>MAAQHGAPPSARSPRFGVNYTPSNGWFHHWLDFDLDAVRADLDSVAALGFDHVRVFPLWPVFQPNRTLIRPRAVEQLAALTDAAGERGLDVNVDGLQGHLSSFDFLPAWTTTWHRRNLFTDPDVVSGQAEYLRTLAAALADRPNFLGMTVGNAINQFSGHPHPDPDRVTPEQAGDWLRRMLDACERGAPGRLHLHAEYDAAWYLDDHPFTPAHSARIGAVTAVHSWVFNGTAQRYGTRSTATAQHAAYLVELAKAWAREPRRPVWLQEVGAPAPHVPAEY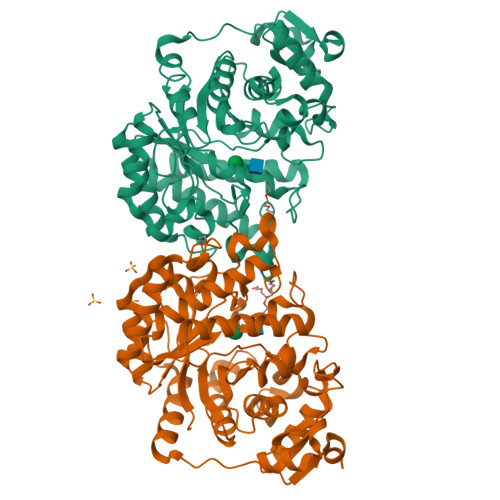AAEFATATIDAVLDCPEVWGVTWWCSHDVDRRLADFPELEYSLGLLTQDRRVKPAGRAVAEAVRRWRTETPAPRPRTTALVVDVGPGDQAPARSVCAPGGAVFEAFMRLTAQGARPTTVLAEHATDADHLAARGITEVVTPHDVHLEHHHHHH[2x]> EL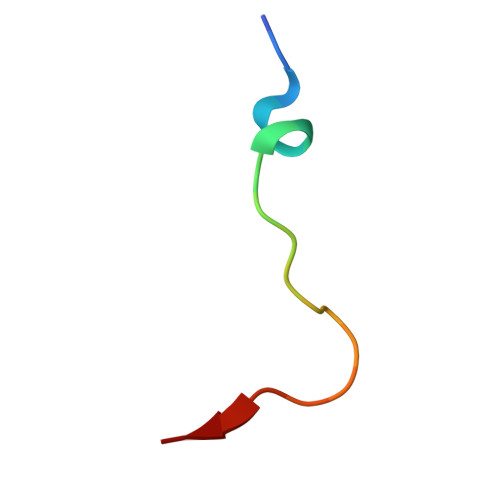DLETLAPYIPMDGEDFQL> EVANPEHYIKHPLQNRWALWFFKNDKSKTWQANLRLISKFDTVEDFWALYNHIQLSSNLMPGCDYSLFKDGIEPMWEDEKNKRGGRWLI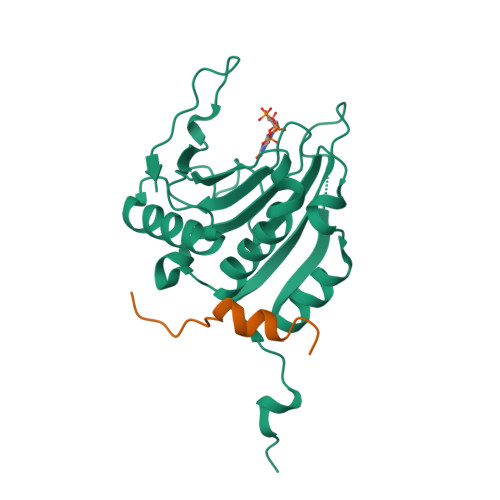TLNKQQRRSDLDRFWLETLLCLIGESFDDYSDDVCGAVVNVRAKGDKIAIWTTECENREAVTHIGRVYKERLGLPPKIVIGYQSHADTATKSGSTTKNRFVV;> PGGTRIIYDRKFLLDRRNS>[8x]MPREIITLQLGQCGNQIGFEFWKQLCAEHGISPEGIVEEFATEGTDRKDVFFYQADDEHYIPRAVLLDLEPRVIHSILNSPYAKLYNPENIYLSEHGGGAGNNWASGFSQGEKIHEDIFDIIDREADGSDSLEGFVLCHSIAGGTGSGLGSYLLERLNDRYPKKLVQTYSVFPNQDEMSDVVVQPYNSLLTLKRLTQNADCVVVLDNTALNRIATDRLHIQNPSFSQINQLVSTIMSASTTTLRYPGYMNNDLIGLIASLIPTPRLHFLMTGYTPLTTDQSVASVRKTTVLDVMRRLLQPKNVMVSTGRDRQTNHCYIAILNIIQGEVDPTQVHKSLQRIRERKLANFIPWGPASIQVALSRKSPYLPSAHRVSGLMMANHTSISSLFERTCRQYDKLRKREAFLEQFRKEDMFKDNFDEMDTSREIVQQLIDEYHAATRPDYISWGTQEQ;>MSEFRIHHDVNELLSLLRVHGGDGAEVYIDLLQKNRTPYVTTTVSAHSAKVKIAEFSRTPEDFLKKYDELKSKNTRNLDPLVYLLSKLTEDKETLQYLQQNAKERAELAAAAVGSSTTSINVPAAASKISMQELEELRKQLGSVATGSTLQQSLELKRKMLRDKQNKKNSGQHLPIFPAWVYERPALIGDFLIGAGISTDTALPIGTLPLASQESAVVEDLLYVLVGVDGRYVSAQPLAGRQSRTFLVDPNLDLSIRELVHRILPVAASYSAVTRFIEEKSSFEYGQVNHALAAAMRTLVKEHLILVSQLEQLHRQGLLSLQKLWFYIQPAMRTMDILASLATSVDKGECLGGSTLSLLHDRSFSYTGDSQAQELCLYLTKAASAPYFEVLEKWIYRGIIHDPYSEFMVEEHELRKERIQEDYNDKYWDQRYTIVQQQIPSFLQKMADKILSTGKYLNVVRECGHDVTCPVAKEIIYTLKERAYVEQIEKAFNYASKVLLDFLMEEKELVAHLRSIKRYFLMDQGDFFVHFMDLAEEELRKPVEDITPPRLEALLELALRMSTANTDPFKDDLKIDLMPHDLITQLLRVLAIETKQEKAMAHADPTELALSGLEAFSFDYIVKWPLSLIINRKALTRYQMLFRHMFYCKHVERQLCSVWISNKTAKQHSLHSAQWFAGAFTLRQRMLNFVQNIQYYMMFEVMEPTWHILEKNLKSASNIDDVLGHHTGFLDTCLKDCMLTNPELLKVFSKLMSVCVMFTNCMQKFTQSMKLDGELGGQTLEHSTVLGLPAGAEERARKELARKHLAEHAD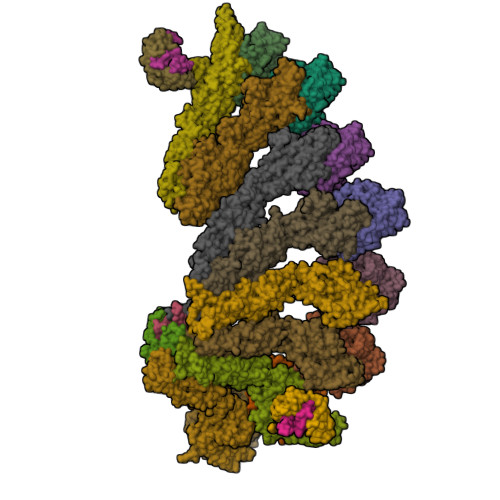TVQLVSGFEATINKFDKNFSAHLLDLLARLSIYSTSDCEHGMASVISRLDFNGFYTERLERLSAERSQKATPQVPVLRGPPAPAPRVAVTAQ[2x];>MATPDQKSPNVLLQNLCCRILGRSEADVAQQFQYAVRVIGSNFAPTVERDEFLVAEKIKKELIRQRREADAALFSELHRKLHSQGVLKNKWSILYLLLSLSEDPRRQPSKVSSYATLFAQALPRDAHSTPYYYARPQTLPLSYQDRSAQSAQSSGSVGSSGISSIGLCALSGPAPAPQSLLPGQSNQAPGVGDCLRQQLGSRLAWTLTANQPSSQATTSKGVPSAVSRNMTRSRREGDTGGTMEITEAALVRDILYVFQGIDGKNIKMNNTENCYKVEGKANLSRSLRDTAVRLSELGWLHNKIRRYTDQRSLDRSFGLVGQSFCAALHQELREYYRLLSVLHSQLQLEDDQGVNLGLESSLTLRRLLVWTYDPKIRLKTLAALVDHCQGRKGGELASAVHAYTKTGDPYMRSLVQHILSLVSHPVLSFLYRWIYDGELEDTYHEFFVASDPTVKTDRLWHDKYTLRKSMIPSFMTMDQSRKVLLIGKSINFLHQVCHDQTPTTKMIAVTKSAESPQDAADLFTDLENAFQGKIDAAYFETSKYLLDVLNKKYSLLDHMQAMRRYLLLGQGDFIRHLMDLLKPELVRPATTLYQHNLTGILETAVRATNAQFDSPEILRRLDVRLLEVSPGDTGWDVFSLDYHVDGPIATVFTRECMSHYLRVFNFLWRAKRMEYILTDIRKGHMCNAKLLRNMPEFSGVLHQCHILASEMVHFIHQMQYYITFEVLECSWDELWNKVQQAQDLDHIIAAHEVFLDTIISRCLLDSDSRALLNQLRAVFDQIIELQNAQDAIYRAALEELQRRLQFEEKKKQREIEGQWGVTAAEEEEENKRIGEFKESIPKMCSQLRILTHFYQGIVQQFLVLLTTSSDESLRFLSFRLDFNEHYKAREPRLRVSLGTRGRRSSHT[4x];>MIHELLLALSGYPGSIFTWNKRSGLQVSQDFPFLHPSETSVLNRLCRLGTDYIRFTEFIEQYTGHVQQQDHHPSQQGQGGLHGIYLRAFCTGLDSVLQPYRQALLDLEQEFLGDPHLSISHVNYFLDQFQLLFPSVMVVVEQIKSQKIHGCQILETVYKHSCGGLPPVRSALEKILAVCHGVMYKQLSAWMLHGLLLDQHEEFFIKQGPSSGNVSAQPEEDEEDLGIGGLTGKQLRELQDLRLIEEENMLAPSLKQFSLRVEILPSYIPVRVAEKILFVGESVQMFENQNVNLTRKGSILKNQEDTFAAELHRLKQQPLFSLVDFEQVVDRIRSTVAEHLWKLMVEESDLLGQLKIIKDFYLLGRGELFQAFIDTAQHMLKTPPTAVTEHDVNVAFQQSAHKVLLDDDNLLPLLHLTIEYHGKEHKADATQAREGPSRETSPREAPASGWAALGLSYKVQWPLHILFTPAVLEKYNVVFKYLLSVRRVQAELQHCWALQMQRKHLKSNQTDAIKWRLRNHMAFLVDNLQYYLQVDVLESQFSQLLHQINSTRDFESIRLAHDHFLSNLLAQSFILLKPVFHCLNEILDLCHSFCSLVSQNLGPLDERGAAQLSILVKGFSRQSSLLFKILSSVRNHQINSDLAQLLLRLDYNKYYTQAGGTLGSFGM[2x];>[2x]MARHGPPWSRLDAQQERDVRELVRGVAGLQDEADPNFQLALNFAWSNFRFHRFLDVNSHKIEKTIEGIYEKFVIHSDLSKAASWKRLTEEFLNAPLPSIKEIKTDAHYSILSLLLCLSDSPSNSSYVETPRNKEVEKKDDFDWGKYLMEDEEMDIGPYMDTPNWSEESEEENDQQPLSREDSGIQVDRTPLEEQDQNRKLDPCISWKDEPDDRSWLEHHVVHQYWTARPSQFPHSLHLHSNLAAVWDQHLYSSDPLYVPDDRVLVTETQVIRETLWLLSGVKKLFIFQLIDGKVTVRNNIIVTHLTHSCLRSVLEQIAAYGQVVFRLQEFIDEVMGHSSESMLPGSGSVPKKSTEAPFRTYQAFMWALYKYFISFKEELAEIEKCIINNDTTITLAIVVDKLAPRLSQLKVLHKVFSTGVAEVPPDTRNVVRASHLLNTLYKAILEYDNVGEASEQTVSLLFSLWVETVRPYLQTVDEWIVHGHLWDGAREFIIQRNKNVPVNHRDFWYATYTLYSVSEKTENEEKMSDNASASSGSDQGPSSRQHTMVSFLKPVLKQIIMAGKSMQLLKNLQCAESTTCQAGARDAERKSLYTLFLESVQSRLRHGEDSTPQVLTEQQATKENLMKMQSIAESHLELDDVHDPLLAINFARMYLEQSDFHEKFAGGDVCVDRSSESVTCQTFELTLRSCLYPHIDKQYLDCCGNLMQTLKKDYRLVEYLQAMRNFFLMEGGDTMYDFYTSIFDKIREKETWQNVSFLNVQLQEAVGQRYPEDSSRLSISFENVDTAKKKLPVHILDGLTLSYKVPWPVDIVISLECQKIYNQVFLLLLQIKWAKYSLDVLLFGELVSTAEKPRLKEGLIHEQDTVAQFGPQKEPVRQQIHRMFLLRVKLMHFVNSLHNYIMTRILHSTGLEFQHQVEEAKDLDQLIKIHYRYLSTIHDRCLLREKVSFVKEAIMKVLNLALMFADGWQAGLGTWRMESIEKMESDFKNCHMFLVTILNKAVCRGSFPHLESLALSLMAGMEQS;> MASITQLFDDLCEALLPAAKTHLGQRSVNRKRAKRSLKKVAYNALFTNLFQDETQQLQPDMSKLPARNKILMLSFDLRVGGLGPKADRLEELVEELEAAPCCPLLEVGSVLDLLVQLAGSGPPQVLPRKRDYFLNNKHVGRNVPYSGYDCDDLSVFEMDVQSLISREECLCHSMIQETLQVMEAAPGTGLPTVGLFSFGDPCGDRFERDTRVSLFGALVHSRTYDMDVRLGLPPVPDNADLSGLAIKVPPSVDQWEDEGFQSASNLTPDSQSEPSVTPDVDLWEAALTYEASKRRCWERVGCPPGHREEPYLTEAGRDAFDKFCRLHQGELQLLAGGVLQAPQPVLVKECELVKDVLNVLIGVVSATFSLCQPAQAFVVKRGVHVSGASPESISSLLSEVAEYGTCYTRLSHFSLQPVLDSLYSKGLVFQAFTSGLRRYLQYYRACVLSTPPTLSLLTIGFLFKKLGRQLRYLAELCGVGAVLPGTCGGGPRAAFPTGVKLLSYLYQEALHNCSNEHYPVLLSLLKTSCEPYTRFIHDWVYSGVFRDAYGEFMIQVNHEYLSFRDKLYWTHGYVLISKEVEDCVPVFLKHIAHDIYVCGKTINLLKLCCPRHYLCWSDVPVPRISVIFSLEELKEIEKDCAVYVGRMERVARHSSVSKEEKELRMEIAKQELIAHAREAASRVLSALSDRQMSERMALDARKREQFQRLKEQFVKDQERRQAARQEELDDDFSYARELRDRERRLKSLEEELERKARQALVDHYSKLSAEAARREQKALWRIQRHRLESARLRFLLEDEKHIQEMLKAVSEAHQPQEPPDVLLSVHPQVTSPGPEHPEGGQGCDSGSAEQHSPAWDGWNRPGLLTPQPLKPLAVGAGGRGLQQAEGARPFSDSLSIGDFLPVGPGAEPSVQTGMVPLLEVALQTINLDLPPSAPGEAPAAASTQPSRPQEYDFSTVLRPAVATSPAPGPLQAAECSLGSSGLQLWEDSCGKMDACGSASRETLLPSHPPRRAALEEGSSQPTERLFGQVSGGGLPTGDYASEIAPTRPRWNTHGHVSDASIRVGENVSDVAPTQPRWNTHGHVSNASISLGESVSDVAPTRPRWNIHGHVSNASIRVGENVSDVAPTRPRWNTHGHVSNASIRVGENVSDVAPTRPRWNTHGHVSDASISLGESVSDMAPARPRWNTHGHVSDASISLGESVSDMAPTRPRWNTHGHVSDTSIRVGENVSDVAPIRSRCNTHGHVSDASISLGEPVSDVVSTRPRWNTHVPIPPPHMVLGALSPEAEPNTPRPQQSPPGHTSQSALSLGAQSTVLDCGPRLPVEVGPSLSSPSSGCGEGSISVGENVSDVAPTQPWWPNTPGDSVSEELGPGRSGDTEDLSPNWPLNSQEDTAAQSSPGRGEEAEASAAEAQGGEQAYLAGLAGQYHLERYPDSYESMSEPPIAHLLRPVLPRAFAFPVDPQVQSAADETAVQLSELLTLPVLMKRSITAPLAAHISLVNKAAVDYFFVELHLEAHYEALRHFLLMEDGEFAQSLSDLLFEKLGAGQTPGELLNPLVLNSVLSKALQCSLHGDTPHASNLSLALKYLPEVFAPNAPDVLSCLELRYKVDWPLNIVITEGCVSKYSGVFSFLLQLKLMMWALKDVCFHLKRTALLSHMAGSVQFRQLQLFKHEMQHFVKVIQGYIANQILHVTWCEFRARLATVGDLEEIQRAHAEYLHKAVFRGLLTEKAAPVMNVIHSIFSLVLKFRSQLISQAWGPPGGPRGAEHPNFALMQQSYNTFKYYSHFLFKVVTKLVNRGYQPHLEDFLLRINFNNYYQDA;>MASSSGAGAAAAAAAANLNAVRETMDVLLEISRILNTGLDMETLSICVRLCEQGINPEALSSVIKELRKATEALKAAENMTS[3x]2-{(R)-(3-{[4-(dimethylamino)butanoyl]amino}phenyl)[2-(piperidin-1-yl)ethoxy]methyl}thieno[3,2-b]pyridine-7-carboxylic 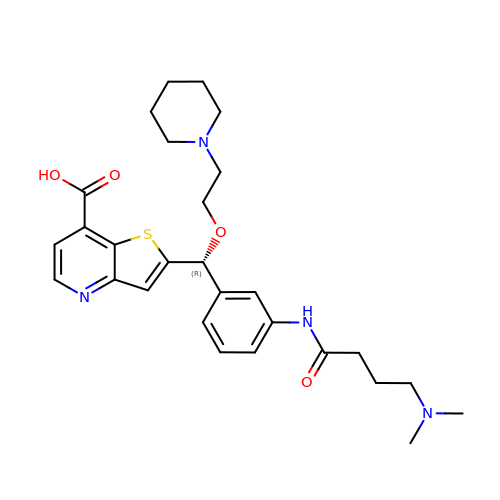acid | C28 H36 N4 O4 S | GTUZDQNWYGEDTB-AREMUKBSSA-N5ALPHA-ANDROSTAN-3,17-DIONE | C19 H28 O2 | 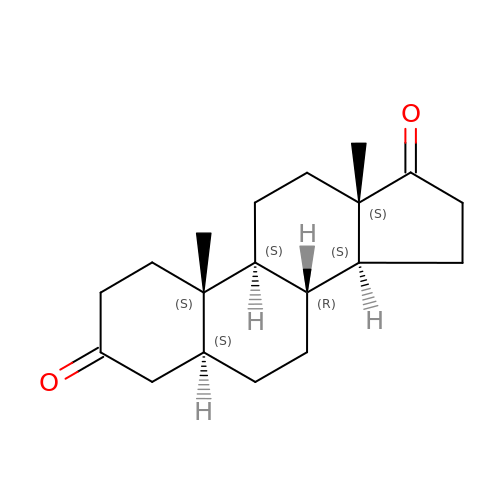RAJWOBJTTGJROA-WZNAKSSCSA-N> GSAGSGTIDDDDKMEKLIVAGPKRLARELLAELQKAGVVHIDPLRPDELGEYRLSPTEEAELKRWEAVVSQAEQSLTVVGLATVPSSKPFTGSLEEAEAVLRPVASRAEVLGKERAALEEEIQTIELFGKAAEKLAALAHGLDESPRLGVIPFLVAKPEELEAVRKALQEALADRFVLEAEPLENQLAALVVVKRSELEAARSSLSRLGLAELRFPGAYGAMPLGKAAARMKERARLAPEELVGIREEVARLSRESGEALIALWTR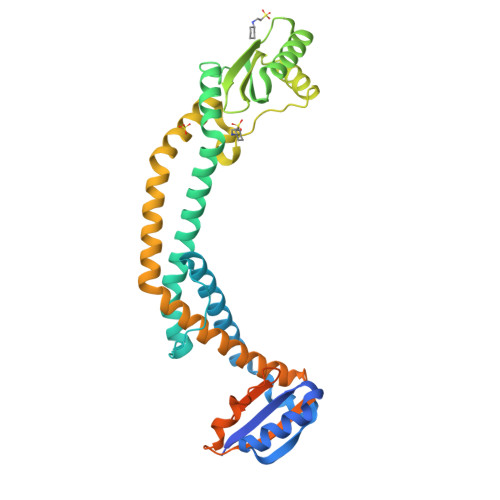AKDEVARYKAVADMAAGKYGAALMGWVPQKAKGKVEEALGRLRDQIVYTFEPVDEHHESHQVPVTLENPAWAKPFELLHGFLNTPAYGSHD> GGIR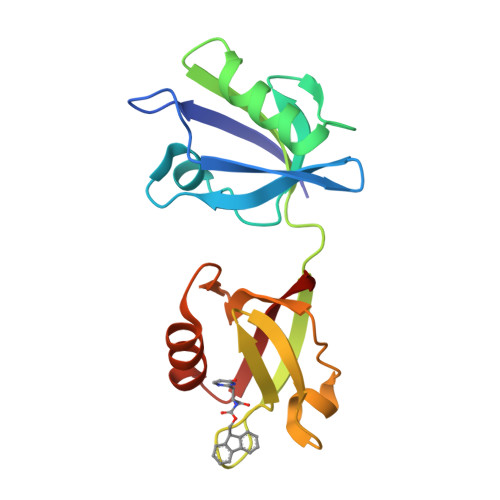EVILCKDQDGKIGLRLKSVDNGIFVQLVQANSPASLVGLRFGDQVLQINGENCAGWSSDKAHKVLKQAFGEKITMTIRDRPFERTVTMHKDSSGHVGFIFKSGKITSIVKDSSAARNGLLTDHHICEINGQNVIGLKDAQIADILSTAGTVVTITIMPA> GGSGGSMPPPADIVKVAIEWPGAYPKLMEIDQKKPLSAIIKEVCDGWSLANHEYFALQHADSSNFY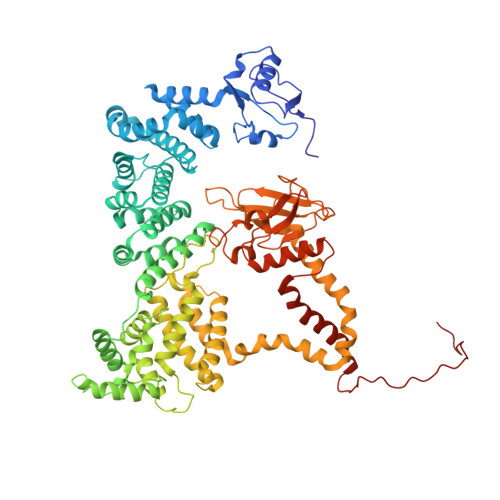ITEKNRNEIKNGTILRLTTSPAQNAQQLHERIQSSSMDAKLEALKDLASLSRDVTFAQEFINLDGISLLTQMVESGTERYQKLQKIMKPCFGDMLSFTLTAFVELMDHGIVSWDTFSVAFIKKIASFVNKSAIDISILQRSLAILESMVLNSHDLYQKVAQEITIGQLIPHLQGSDQEIQTYTIAVINALFLKAPDERRQEMANILAQKQLRSIILTHVIRAQRAINNEMAHQLYVLQVLTFNLLEDRMMTKMDPQDQAQRDIIFELRRIAFDAESEPNNSSGSMEKRKSMYTRDYKKLGFINHVNPAMDFTQTPPGMLALDNMLYFAKHHQDAYIRIVLENSSREDKHECPFGRSSIELTKMLCEILKVGELPSETCNDFHPMFFTHDRSFEEFFCICIQLLNKTWKEMRATSEDFNKVMQVVKEQVMRALTTKPSSLDQFKSKLQNLSYTEILKIRQSERMNQEDFQSRPILELKEKIQPEILELIKQQRLNRLVEGTCFRKLNARRRQDKFWYCRLSPNHKVLHYGDLEESPQGEVPHDSLQDKLPVADIKAVVTGKDCPHMKEKGALKQNKEVLELAFSILYDSNCQLNFIAPDKHEYCIWTDGLNALLGKDMMSDLTRNDLDTLLSMEIKLRLLDLENIQIPDAPPPIPKEPSNYDFVYDCN>[2x]KPAPSTIFSPEKALGLLLSLKLSKWQYITLRETTIREGSKEIYPSYYKVQKAKLQCYPPKAFVAVTDSSAKIALQALLDLTVNRIFETIRSPDAIQNKQLILISKWGFDGASNQSRYKQNIESGQGDS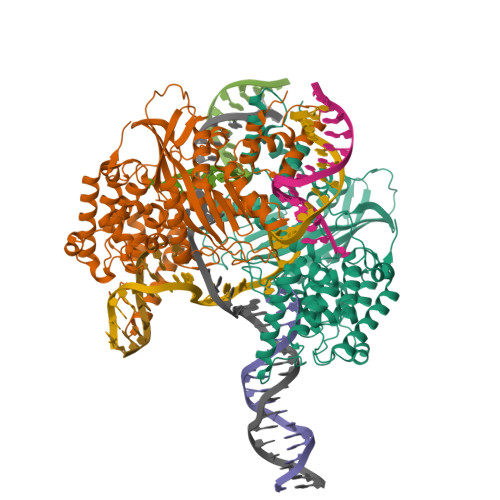SIFMTSLVPLKLTADGDTVWVNPKPCSPMYCRPVQFSFVKETKDVVINEKTAMDDEIEALVPSKCQGHEISHKLMMTMIDGKICTYLSEAKSNAACYLCLAKPTEMSKLDVIASKTISSGVYEFGLSTLHARINVMECLLHIAYRLDFKKWSARGEGHQELLHSRKKLIQDRFKDDLNLLIDIVKQGSGTTNDGNTARRFFEFPDKTAAITGLDEDLIRRFSVILQAITSGEIIDVPKFKEYARTTAEKYVELYDWYYMSSTVHKLLIHGGDIIAENAIVPIGSLSEEASEARNKDFRRFREHHSRKKSRQASNEDILNMLIISSDPLISFTRPKLDAHKRQTYFKETVELLQLQDQEAPTEFHHHHHH>[2x]MASFSSYANGVKRWYQKLELPMPPERIFGAHMMLIGGLACLIGTYFFASMTMWNDGYVNLTLRPRLISLGIYDPYDTEQIQRVWLPLIGEFSTSKLPFFGQYPLTMTDFRLFGWGCFHIGLGLWLVYAGAAHYYGARGGATIGEIFWLLPYVPGLKGLCQIKWFTPEGPWYKVGLPWGSFANTPWPILRRTYADALSPHTIYIGLLFFIWGFVLWFVLDKPPVPLQPAQVMTPNGLMPLEQAPFPYGWFDPYLNQVMHPMNTINGETTMCFVWGVLFVALGAYWWYRPPRSINITHLEDTKAVFHVHLTAIGYVSFALAIVGFLALRNHPSYLMLNDMNVIIYGKKIVNPGRMIHNMITFNHVQVGLLYVAAG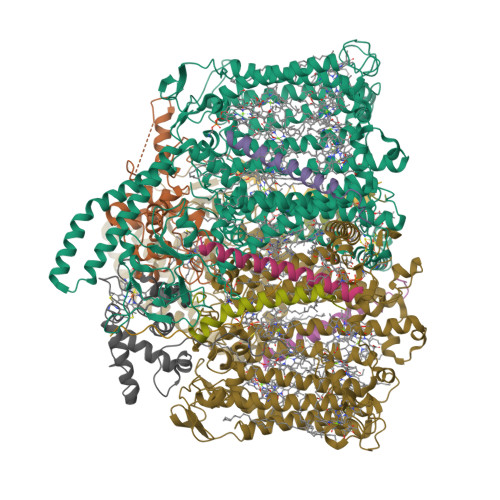VFHGGQYLHGLNISGAYKQARSKFITWFQNPDLQTKIVGTTMFVSFVTVVFGYGMICWNTGAELDLNFGIYQFRSFRAIQMDGEAGNIGYRVFRPKNPWDPTAGGDWVKNPDGTAKLVKARNLQVGDRILNEELGIGSSPTYSFTTIEEINYKPEWGQPKLYAVQWGSWTHFLRKVNPLFWVDKGIWYLQNQKTFEATRKADEAYLAAHLKAVSLLNQIDDAQTEEAKQKAQAELDKFRPELEKAHANMLEWNERLASTPAVLYSNLRDQHRDGEINDAIFFWLMIGGWLFGFIPLLRIAFHNYQSPWYRDFEWRKQSPDFPCIGPVKGGTCGVSIQDQLWFCILFSIKPLSAIAWYLDGGWIATMMARGNEAYYLTHNISHTGGVFLYMWNETTWIWTDNHLTAMLLLGHLIWFVSFALWFKDRGSRAEGGDIQSRWVRLMGKRLGIKTLQEVRFPVSNLATAKLWGTVFFYTGTFVLVFLYFADGFFQNR;> MKSIKIIVLGSALALLVGGCFVGSRDPNETRYPKAPMPLQNQTSTLKTAEEIRRESVAQNTPGAREAAALRDRVTPLNLQQVNEQDVAGNDPLGSPARVVLDEGEMYRDPVEIYREGRALFQNNCVGCHGHNGCGNVPRSTNFTDPGWQENNSDGGIYSSIYNGKGIGNGGGAMPAYYNQLSPQQIRYLVAYLRAFKGRQCNGLPTLSDVERMVAERQNKP;>[2x]MTAILLACLFVLGGYAALWGIIKFVVANTKDIAAN;>[2x]MWNVVGQIISVLCFFILTVGTLFGIVYVSHLLSRG;>MEGVAMEDISKVAWAWFGVLLAICLIGAFGNYVPKLFVKMLMFLN[2x];> VMATGCFVGARNASEPRLGSSSIAASRTAPAYLREAQVLYEGSTDGLPKDTPADEIAHYKAMLAELQTRNYAACAGCHQVNGGGNKAINATNFQDAGWQANNSSPGMVTSIVNGKGKVMPAYKDKLTLQQINYLVEYIRRFEKKR>[2x]MGHHHHHHHHHHSSGYHIQGRHMQRINALTIAGTDPSGGAGIQADLKTFSALGAYGCSVITALV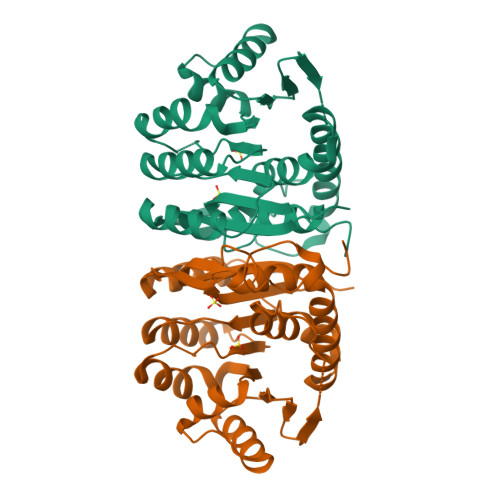AENTCGVQSVYRIEPDFVAAQLDSVFSDVRIDTTKIGMLAETDIVEAVAERLQRHHVRNVVLDTVMLAKSGDPLLSPSAIETLRVRLLPQVSLITPNLPEAAALLDAPHARTEQEMLAQGRALLAMGCEAVLMKGGHLEDAQSPDWLFTREGEQRFSAPRVNTKNTHGTGCTLSAALAALRPRHRSWGETVNEAKAWLSAALAQADTLEVGKGIGPVHHFHAWW>GHMDEPTA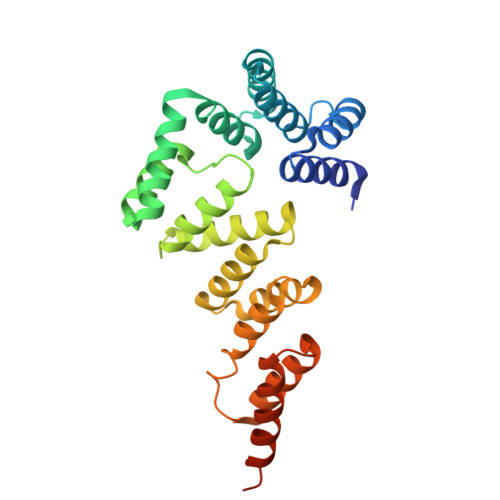QQQLLSQVRLGEATKREDLVRQSLYRLELIDPDNPDVIAARFRYLLRQGDNAGAQKQLDRMKQLAPDSAAYKSSVTSMTLSGAEGRQALQQARLQATTGHVPEALAAYDALFKGNPPEGDLAVEYWALVAKVPARRSEAITQLKALNARNPGNAALQNSLAQLLFGEGRDAEAYAVLEQMAKSSAGREAAAGLWYQQIQRMPVSDASVKALQRFLTVFSSGDTVDSARTQLAAQQKQLADPAFRLEHHHHHH[5x]>[4x]ANPCCSNPCQNRGECMSTGFDQYKCDCTRTGFYGENCTTPEFLTRIKLLLKPTPNTVHYILTHFKGVWNIVNNIPFLRSLIMKYVLTSRSYLIDSPPTYNVHYGYKSWEAFSNLSYYTRALPPVADDCPTPMGVKGNKELPDSKEVLEKVLLRREFIPDPQGSNMMFAFFAQHFTHQFFKTDHKRGPGFTRGLGHGVDLNHIYGETLDRQHKLRLFKDGKLKYQVIGGEVYPPTVKDTQVEMIYPPHIPENLQFAVGQEVF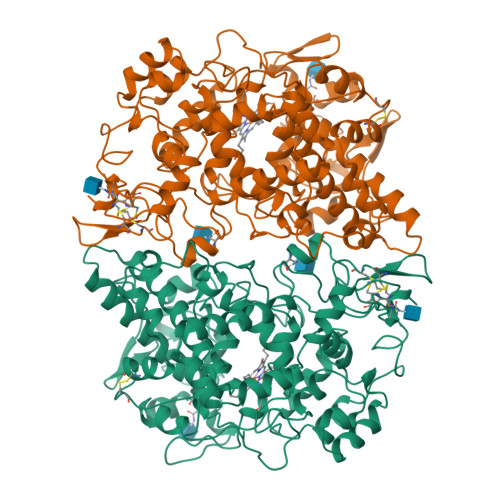GLVPGLMMYATIWLREHQRVCDILKQEHPEWGDEQLFQTSKLILIGETIKIVIEDYVQHLSGYHFKLKFDPELLFNQQFQYQNRIASEFNTLYHWHPLLPDTFNIEDQEYSFKQFLYNNSILLEHGLTQFVESFTRQIAGRVAGGRNVPIAVQAVAKASIDQSREMKYQSLNEYRKRFSLKPYTSFEELTGEKEMAAELKALYSDIDVMELYPALLVEKPRPDAIFGETMVELGAPFSLKGLMGNPICSPQYWKPSTFGGEVGFKIINTASIQSLICNNVKGCPFTSFNVQDPQPTKTATINASASHSRLDDINPTVLIKRRSTEL> GSGSELWRQCTHWLIQCRVLPPSHRVTWDGAQVCELAQALRDGVLLCQLLNNLLPHAINLREVNLRPQMSQFLCLKNIRTFLSTCCEKFGLKRSELFEAFDLFDVQDFGKVIYTLSALSWTPIAQNRGIMPFPTEEESVGDEDIYSGLSDQIDDTVEEDEDLYDCVENEEAE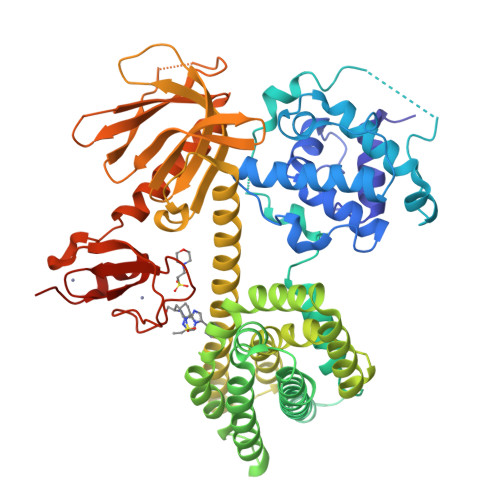GDEIYEDLMRSEPVSMPPKMTEYDKRCCCLREIQQTEEKYTDTLGSIQQHFLKPLQRFLKPQDIEIIFINIEDLLRVHTHFLKEMKEALGTPGAANLYQVFIKYKERFLVYGRYCSQVESASKHLDRVAAAREDVQMKLEECSQRANNGRFTLRDLLMVPMQRVLKYHLLLQELVKHTQEAMEKENLRLALDAMRDLAQCVNEVKRDNETLRQITNFQLSIENLDQSLAHYGRPKIDGELKITSVERRSKMDRYAFLLDKALLICKRRGDSYDLKDFVNLHSFQVRDDSSGDRDNKKWSHMFLLIEDQGAQGYELFFKTRELKKKWMEQFEMAISNIYPENATANGHDFQMFSFEETTSCKACQMLLRGTFYQGYRCHRCRASAHKECLGRVPPCGRHGQDFPGTM>[2x]YVMAIDQGTTSSRAIIFDRNGKKIGSSQKEFPQYFPKSGWVEHNANEIWNSVQSVIAGAFIESGIRPEAIAGIGITNQRETTVVWDKTTGQPIANAIVWQSRQSSPIADQLKVDGHTEMIHEKTGLVIDAYFSATKVRWLLDNIEGAQEKADNGELLFGTIDSWLVWKLTDGQVHVTDYSNASRTMLYNIHKLEWDQEILDLLNIPSSMLPEVKSNSEVYGHTRSYHF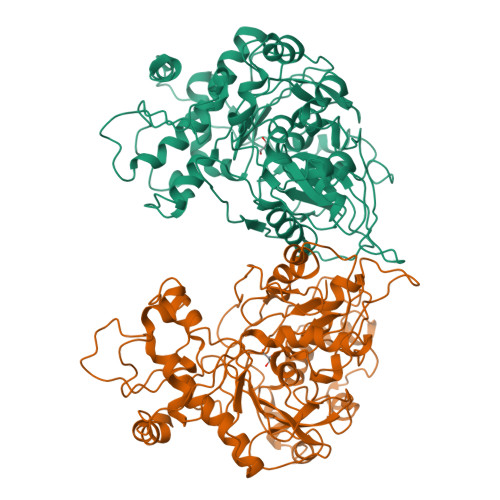YGSEVPIAGMAGDQQAALFGQMAFEKGMIKNTYGTGAFIVMNTGEEPQLSDNDLLTTIGYGINGKVYYALEGSIFVAGSAIQWLRDGLRMIETSPQSEELAAKAKGDNEVYVVPAFTGLGAPYWDSEARGAVFGLTRGTTKEDFVRATLQAVAYQSKDVIDTMKKDSGIDIPLLKVDGGAAKNDLLMQFQADILDIDVQRAANLETTALGAAYLAGLAVGFWKDLDELKSMAEEGQMFTPEMPAEERDNLYEGWKQAVA>[2x]VGLTTLFWLGAIGMLVGTLAFAWAGRDAGSGERRYYVTLVGISGIAAVAYVVMALGVGWVPVAERTVFAPRYIDWILTTPLIVYFLGLLAGLDSREFGIVITLNTVVMLAGFAGAMVPGIERYALFGMGAVAFLGLVYYLVGPMTESASQRSSGIKSLYVRLRNLTVILWAIYPFIWLLGPPGVALLTPTVDVALIVYLDLVTKVGFGFIALDAAATLRAEHGESLAGVDTDAPAVADENSHHHHHHH;>AVSRLLLPSRVRHSYTGKMGAVFIFVGALTVLFGAIAYGEVTAAAATGDAAAVQEAAVSAILGLIILLGINLGLVAATLFGDTAASLSTLAAKASRMGDGDLDVELETRREDEIGDLYAAFDEMRQSVRTSLEDHHHHHHH[2x]

The photoreceptor sensory rhodopsin II from N. pharaonis (NpSRII) in complex with its cognate transducer NpHtrII serves as a model system for studying transmembrane signal transfer. This complex displays a 2:2 stoichiometry where two transducers are flanked by two receptors. The long rod-shaped cytoplasmic domain consists of two HAMP domains (present in Histidine kinases, Adenyl cyclases, Methyl-accepting proteins and Phosphatases23), which are followed by a methylation domain4 involved in the adaptation processes and a signaling domain which harbors the CheW/CheA binding site5. HAMP subunits contain two amphiphilic helices (AS1 and AS2) joined by a non-helical connector.

In this state, the HAMP domain adopts a compact conformation which has been correlated with the active state of the complex. This conformational state is made possible by a high flexibility of the linker, especially in the region of Gly83-Gly84 amino acid repeat. Indeed, replacing a small glycine by a considerably larger phenylalanine would limit the ability of the HAMP domain to rotate relative to the membrane part of the transducer and thus forbids the ground state. In line with this reasoning, our data on the crystal structure of the NpSRII/NpHtrII1–135-G83F mutant demonstrate different crystal packing. Although the crystallization conditions were the same as for the wild type “U”-shaped complex in the P64 space group, in this case the space group is P21212 giving the “V”-shape structure similar to those observed before. The previously published X-Ray diffraction data on the NpSRII/NpHtrII complex only showed electron densities for the transmembrane domain of the transducer but not for its adjacent HAMP domain. These crystals of the wild type NpSRII in complex with the shortened NpHtrII (NpHtrII1–157 and NpHtrII1–114) belonging to the space group P21212 revealed an overall “V”-shaped topology with an opening to the cytosplasmic side. In the previously determined structure of the complex (space group P21212) quaternary structure has a “V”-shape and there was no possibility of interaction between the NpHtrII’s HAMP1 domain and NpSRII.> GAMETLHITKTMKNIEVPETKTASFECEVSHFNVPSMWLKNGVEIEMSEKFKIVVQGKLHQLIIMNTSTEDSAEYTFVCGNDQVSATLTV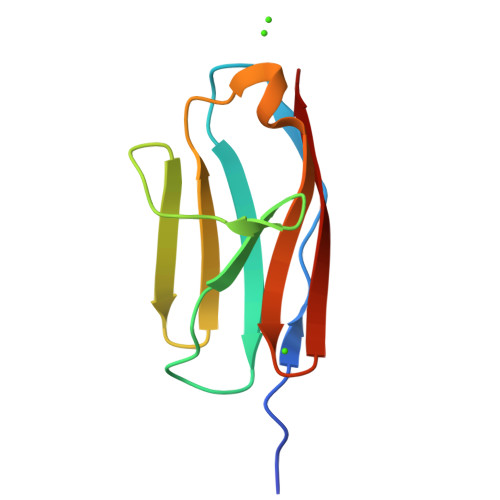T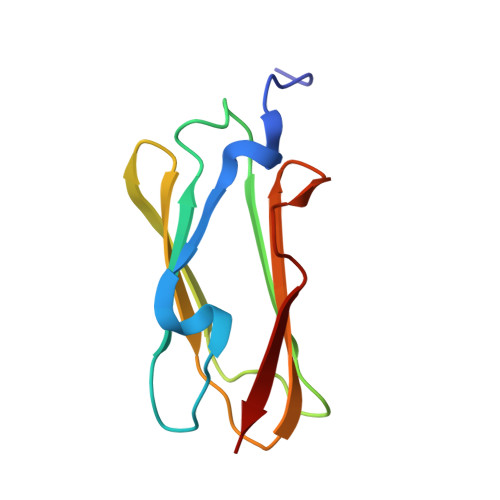> GSKFSSDASKVVTRGPGLSQAFVGQKNSFTVDCSKAGTNMMMVGVHGPKTPCEEVYVKHMGNRVYNVTYTVKEKGDYILIVKWGDESVPGSPFKVKVP> METACERLHVAQETQMQLIEKSSDKLQDHILYWTAVRTENTLLYAARKKGVTVLGHCRVPHSVVCQERAKQAIEMQLSLQELSKTEFGDEPWSLLDTSWDRYMSEPKRCFKKGARVVEVEFDGNASNTNWYTVYSNLYMRTEDGWQLAKAGADGTGLYYCTMAGA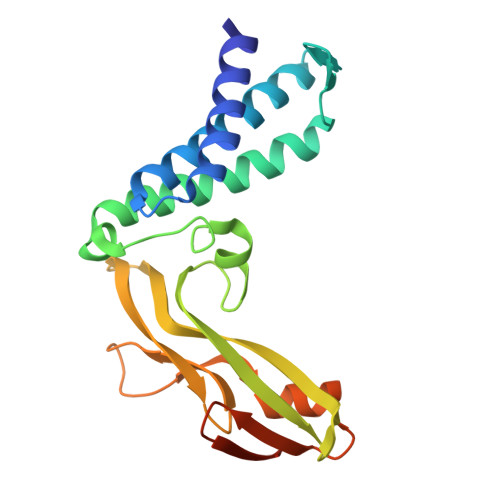GRIYYSRFGDEAARFSTTGHYSVRDQDRVYAGVSSTSSDFRDRP> NKTHQVEHESEQSDFQDIRFGLNSVKLPKAQPAAATRITVENGTDKLVNYKSSPQQLFLAKNALKDKLQGEFDKFLSDAKAFPALTADLQEWVDQQLFNPNQSFFDLSAPRSNFTLSSDKKASLDFIFRFTNFTESVQLLKLPEGVSVVVDSKQSFDYYVNASAQKLLVLPLSLPDYTLGLNYMFDHITLNGKVVNKFSFNPFKTNLNLAFSNVYNGVDVFEAQKNLVGKGKYLNTHVKAEDVKKDVNANIKNQFDIAKIIAELMGKALKEFGNQQEGQPLSFLKVMDKVKEDFEKLFNLVRPGLGKFVKDLIQSSSQAENKITVYKLIFDNKKTILNLLKELSIPELNSSLGLVDVLFDGITDSDGLYERLQSFKDLIVPAVKTNEKTAALSPLIEELLTQKDTYVFDLIQKHKGILTNLLKNFLADFQKSTPFMADQVAIFTELFDNEGAFDLFGEADFVDKIAELFLTKRTVKNGEKIETKDSLLVTSLKSLLGEKVAALGDLLDSYIFKNELLNRSVEVAKAEAKDTKGATDYKKEQAKALKKLFKHIGENTLSKTNLDKITLKEVKNTENVELEETETTLKVKKLDVEYKVELGNFEIKNGLIKAMLEFLPDTKDLETTLDKLLFKGESYKAMKDKYIKEGFPGYGWAKGVVPGAFESIENTFKSAIDKTKSIRDLFGDMLFGNDLSSVKETDSFITLGGSFDIKYGGENLNVLPAYYSLINSEIGYQIIGVDTTIDATKVKVELKNKEYKGKSPAINGQVKLSQSFFNVWTNMFDSITKQIFQKKYEFKDNIQVFARNEDNTSRLELDISDPEQRVIPFAFVDGFGIQLKAVDKNITKEAGNTEPKSPVIQLYEALNKEKDQKQQSKQSPKQLDTKTQLGYLLKLGDNWSKDDYKSLIDD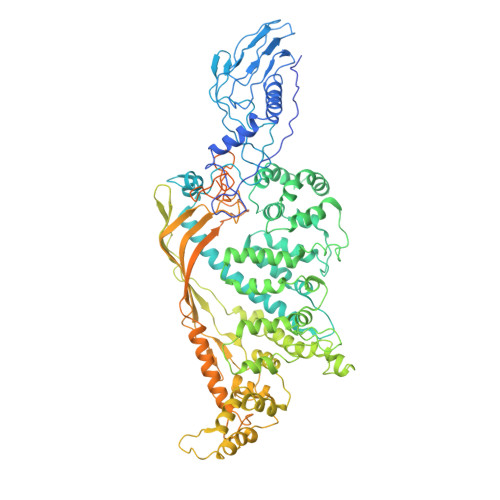TIINNNYLEASFNSKITVDRLGIPIDLWLFKIWPKFNLEIPMQGSLQLYSSSVIFPYGIYDTSVQDAAKIVKRLNFTDMGFKLNDPKPNFWFVGFKHHHHH N-[(benzyloxy)carbonyl]-L-histidyl-N-methyl-L-phenylalanyl-N-hydroxy-L-tryptophanamide 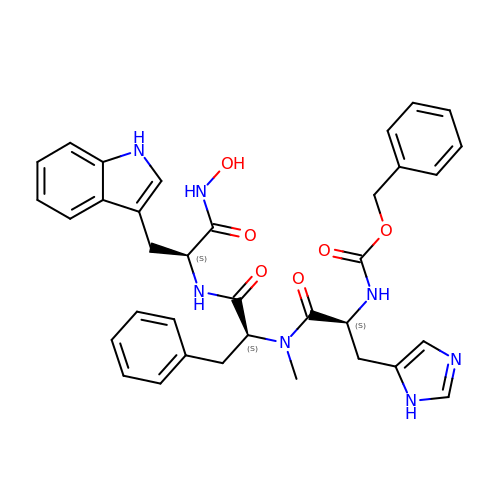| C35 H37 N7 O6 | PUYLOEIRYPDFJO-CHQNGUEUSA-N>[12x]GPLGSPEFRYFVAMFDYDPSTMSPNPDGCDEELPFQEGDTIKVFGDKDADGFYWGELRGRRGYVPHNMVSEVE;>XTRRRRKLPEIPKNKKX[12x]

RBP, via its second and third SH3 domain, is known to bind synaptic ligands such as Ca2+ channels and RIM. Drosophila RBP SH3-II and -III share 49.2% sequence identity and adopt the canonical fold of SH3 domains. We observed the classical poly-proline helix that allows for mainly hydrophobic protein-peptide interaction in all three structures. In summary, we find that the SH3-II and -III interaction surface of RBP serves as a multi-functional platform for differential protein interaction with either other AZ components or the transport adaptor and therefore, motor-cargo linkage.

Finally, in order to get a deeper atomic insight into the structural basis of the binding of RBP towards Aplip1 in comparison to its synaptic ligands, we crystallized the Drosophila RBP SH3-II domain together with both an Aplip1 and a Cac peptide, and RBP SH3-III with a Cac peptide. We detected the same hydrogen pattern between the protein side chains and peptide backbone in the structure of SH3-II with Aplip1 and Cac. The equivalent residue to R1687 of Cac is R153 of the Aplip1 peptide, which forms, by contrast, a bidentate salt-bridge to D1336. Whereas the C-terminal portion of the Aplip1 peptide is folded in a short 310 helix, the N-terminus of the Aplip1 peptide adopts a random coil conformation with hydrophobic interactions to the surface of SH3-II. Completeness of the model given for the 12 complexes of RBP SH3-II bound to the Aplip1 peptide 149TRRRRKLPEIPKNKK163. Whereas we could not detect any binding of the Aplip1 peptides to RBP SH3-I, we could determine KD constants for the single SH3-II, SH3-III and the tandem SH3-II+III domains of RBP. Both SH3-II and SH3-III single domains showed a binding affinity to Aplip1 peptides several fold stronger compared to either Cac, RIM1 or RIM2 (Figure 3—figure supplements 2–4). Aplip1 showed the strongest interaction with RBP compared with Cacophony (Cac), RIM1 and RIM2, with the strongest affinity (lowest KD) between Aplip1 and the RBP SH3-II+III domain. Notably, the same RBP SH3 domain (II and III) interaction surfaces are used for binding the synaptic AZ ligands of RBP, that is, RIM and the voltage gated Ca2+ channel, though with clearly lower affinity than for Aplip1. A point mutation which disrupts the Aplip1-RBP interaction provoked a ‘premature’ capture of RBP and the co-transported BRP at the axonal membrane, thus forming ectopic but, concerning T-bar shape and BRP/RBP arrangement, WT-like AZ scaffolds.>[2x]GHMSPNYDKWEMERTDITMKHKLGGGQYGEVYEGVWKKYSLTVAVKTLKEDTMEVEEFLKEAAVMKEIKHPNLVQLLGVCTREPPFYIITEFMTYGNLLDYLRECNRQEVNAVVLLYMATQISSAMEYLEKKNFIHRDLAARNCLVGENHLVKVADFGLSRLMTGDTYTAPAGAKFPIKWTAPESLAYNKFSIKSDVWAFGVLLWEIATYGMSPYPGIDLSQVYELLEKDYRMERPEGCPEKVYELMRACWQWNPSDRPSFAEIHQAFETMFQESSISDEVEKELGK

BCR–Abl is a constitutively activated form of the nonreceptor tyrosine kinase c-Abl. The improper activation of the Abl tyrosine kinase results in chronic myeloid leukemia (CML). The recognition of an inactive conformation of Abl, in which a catalytically important Asp-Phe-Gly (DFG) motif is flipped by approximately 180° with respect to the active conformation, underlies the specificity of the cancer drug imatinib, which is used to treat CML. Our results suggest that interconversion between distinctly different inactive conformations is a characteristic feature of the Abl kinase domain.

Molecules E and G were obtained from the same crystal form of Abl and are very similar, except for the presence of either the ATP-peptide analog (molecule E) or the kinase inhibitor PD166326 (molecule G). In these structures, the kinase adopts a conformation intermediate between αC-Glu In and αC-Glu Out: while helix αC is not rotated out of the active site of the kinase, a rotation of the side chain of Glu 286 has occurred, resulting in the breakage of the Glu 286–Lys 271 salt bridge. The conformation of Abl represented by molecules E and G suggests a mechanism by which Abl can interconvert between αC-Glu In and αC-Glu Out conformations.>GAMGSSSVWGVAFSPDGQTIASASDDKTVKLWNRNGQLLQTLTGHSSSVWGVAFSPDGQTIASASDDKTVKLWNRNGQLL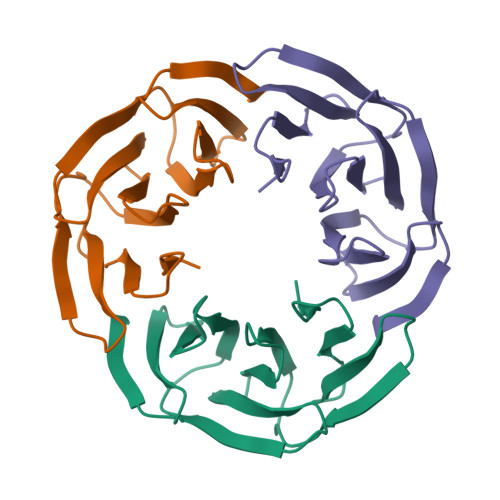QTLTGHSSSVWGVAFSPDGQTIASASDDKTVKLWNRNGQLLQTLTGH[6x]7-(4-fluorophenyl)quinoxalin-5-ol | C14 H9 F N2 O | 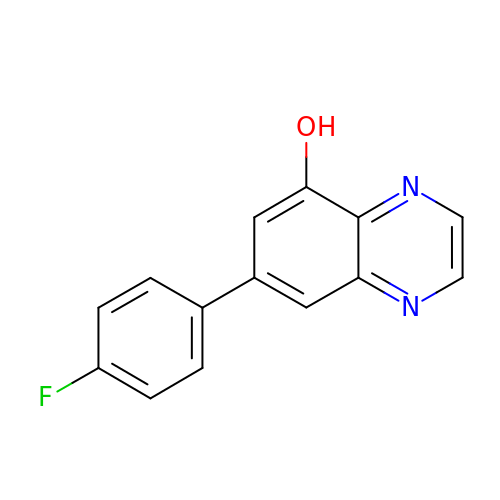YJDUBGAXILBNCU-UHFFFAOYSA-N>[6x]MAPSYKLTYCPVKALGEPIRFLLSYGEKDFEDYRFQEGDWPNLKPSMPFGKTPVLEIDGKQTHQSVAISRYLGKQFGLSGKDDWENLEIDMIVDTISDF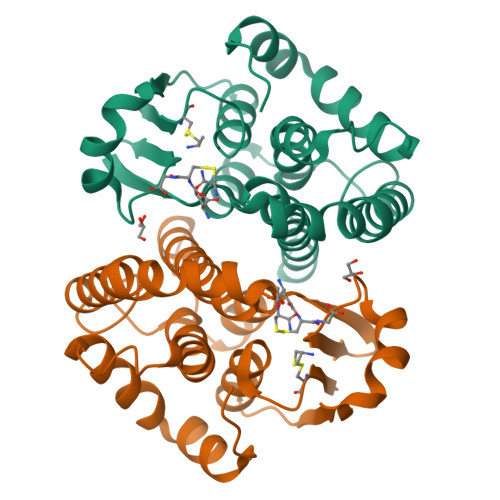RAAIANYHYDADENSKQKKWDPLKKETIPYYTKKFDEVVKANGGYLAAGKLTWADFYFVAILDYLNHMAKEDLVANQPNLKALREKVLGLPAIKAWVAKRPPTDL> IFPKQYPIINFTTAGATVQSYTNFIRAVRGRLTTGADVRHEIPVLPNRVGLPINQRFILVELSNHAELSVTLALDVTNAYVVGYRAGNSAYFFHPDNQEDAEAITHLFTDVQNRYTFAFGGNYDRLEQLAGNLRE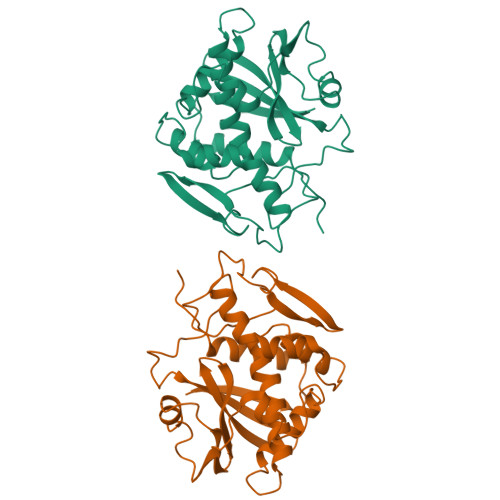NIELGNGPLEEAISALYYYSTGGTQLPTLARSFIICIQMISEAAHFQYIEGEMRTRIRYNRRSAPDPSVITLENSWGRLSTAIQESNQGAFASPIQLQRRNGSKFSVYDVSILIPIIALMVYRCAPPPSSQF> PISPIETVPVKLKPGMDGPKVKQWPLTEEKIKALVEICTEMEKEGKISKIGPENPYNTPVFAIKKKDSTKWRKLVDFRELNKRTQDFWEVQLGIPHPAGLKKKKSVTVLDVGDAYFSVPLDEDFRKYTAFTIPSINNETPGIRYQYNVLPQGWKGSPAIFQSSMTKILEPFKKQNPDIVIYQYMDDLYVGSDLEIGQHRTKIEELRQHLLRWGLTTPDKKHQKEPPFLWMGYELHPDKWTVQPIVLPEKDSWTVNDIQKLVGKLNWASQIYPGIKVRQLCKLLRGTKALTEVIPLTEEAELELAENREILKEPVHGVYYDPSKDLIAEIQKQGQGQWTYQIYQEPFKNLKTGKYARMRGAHTNDVKQLTEAVQKITTE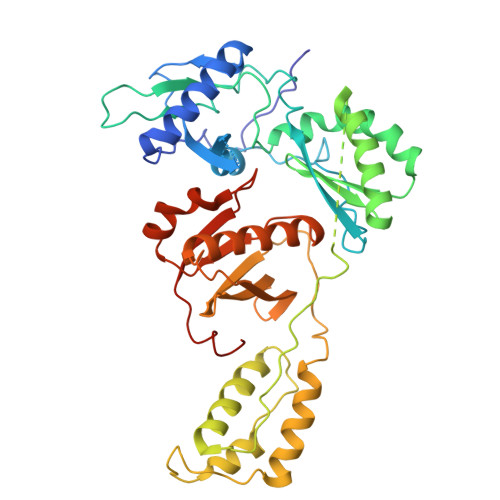SIVIWGKTPKFKLPIQKETWETWWTEYWQATWIPEWEFVNTPPLVKLWYQLEKEPIVGAETF>GHMSDKGKLSLQDVAELIRARACQRVVVMVGAGISTPSGIPDFRSPGSGLYSNLQQYDLPYPEAIFELPFFFHNPKPFFTLAKELYPGNYKPNVTHYFLRLLHDKGLLLRLYTQNIDGLERVSGIPASKLVEAHGTFASATCTVCQRPFPGEDIRADVMADRVPRCPVCTGVVKPDIVFFGEPLPQRFLLHVVDFPMADLLLILGTSLEVEPFASLTEAVRSSVPRLLINRDLVGPLAWHPRSRDVAQLGDVVHGVESLVELLGW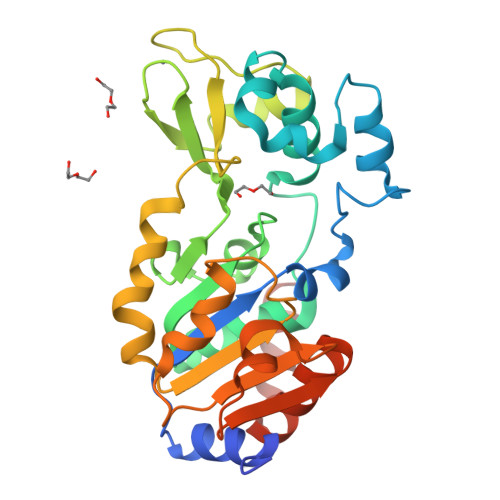TEEMRDLVQRETGKLD[6x]>ARNPITITPQFDCGATNSQQYVARSGDTLTKIAQEIYHDVVGVCDIARANNLADPNRIDAGTPYTIPINCQTYDRNSCL[4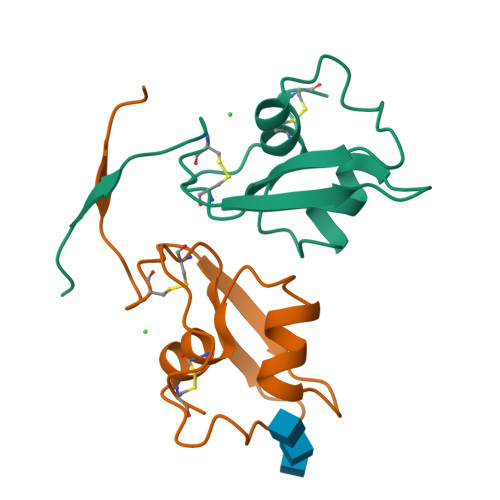x]> 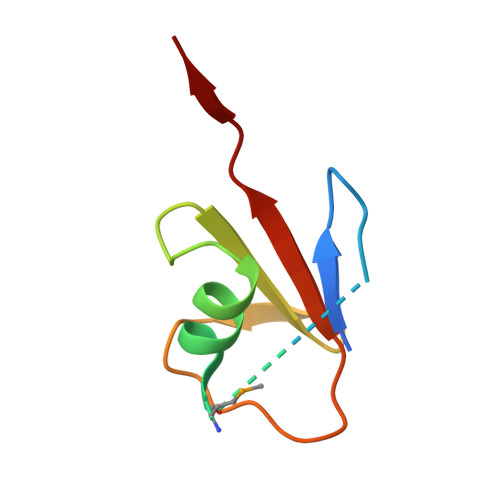MKMIKVKVIGRNIEKEIEWREGMKVRDILRAVGFNTESAIAKVNGKVVLEDDEVKDGDFVEVIPVVSGG> PISPIETVPVKLKPGMDGPKVKQWPLTEEKIKALVEICTEMEKEGKISKIGPENPYNTPVFAIKKKDSTKWRKLVDFRELNKRTQDFWEVQLGIPHPAGLKKNKSVTVLDVGDAYFSVPLDEDFRKYTAFTIPSINNETPGIRYQYNVLPQGWKGSPAIFQSSMTKILEPFRKQNPDIVIYQYMDDLYVGSDLEIGQHRTKIEELRQHLLRWGLTTPDKKHQKEPPFLWMGYELHPDKWTVQPIVLPEKDSWTVNDIQKLVGKLNWASQIYPGIKVRQLCKLLRGTKALTEVIPLTEEAELELAENREILKEPVHGVYYDPSKDLIAEIQKQGQGQWTYQIYQEPFKNLKTGKYARMRGAHTNDVKQLTEAVQKITTESIVIWGKTPKFKLPIQKETWETWWTEYWQATWIPEWEFVNTPPLVKLWYQLEKEPIVGAETFYVDGAANRETKLGKAGYVTNRGRQKVVTLTDTTNQKTELQAIYLALQDSGLEVNIVTDSQYALGIIQAQPDQSESELVNQIIEQLIKKEKVYLAWVPAHKGIGGNEQVDKLVSAGIRKVL;> PISPIETVPVKLKPGMDGPKVKQWPLTEEKIKALVEICTEMEKEGKISKIGPENPYNTPVFAIKKKDSTKWRKLVDFRELNKRTQDFWEVQLGIPHPAGLKKNKSVTVLDVGDAYFSVPLDEDFRKYTAFTIPSINNETPGIRYQYNVLPQGWKGSPAIFQSSMTKILEPFRKQNPDIVIYQYMDDLYVGSDLEIGQHRTKIEELRQHLLRWGLTTPDKKHQKEPPFLWMGYELHPDK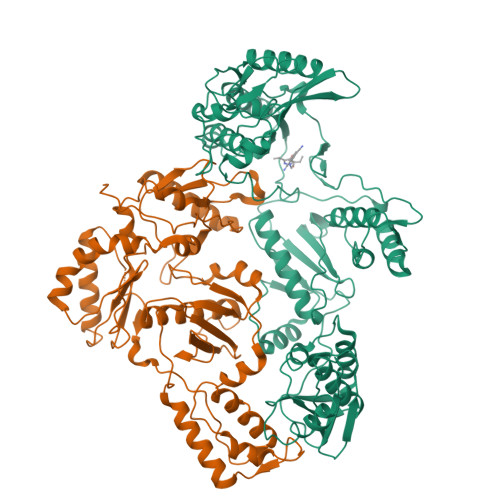WTVQPIVLPEKDSWTVNDIQKLVGKLNWASQIYPGIKVRQLCKLLRGTKALTEVIPLTEEAELELAENREILKEPVHGVYYDPSKDLIAEIQKQGQGQWTYQIYQEPFKNLKTGKYARMRGAHTNDVKQLTEAVQKITTESIVIWGKTPKFKLPIQKETWETWWTEYWQATWIPEWEFVNTPPLVKLWYQLEKEPIVGAETF>MPACCSWNDVFQYETNKVTRIQSVNYGTIKWILHMTVFSYVSFALMSDKLYQRKEPLISSVHTKVKGVAEVTENVTEGGVTKLVHGIFDTADYTLPLQGNSFFVMTNYLKSEGQEQKLCPEYPSRGKQCHSDQGCIKGWMDPQSKGIQTGRCIPYDQKRKTCEIFAWCPAEEGKEAPRPALLRSAENFTVLIKNNIDFPGHNYTTRNILPGMNISCTFHKTWNPQCPIFRLGDIFQEIGENFTEVAVQGGIMGIEIYWDCNLDSWSHRCQPKYSFRRLDDKYTNESLFPGYNFRYAKYYKENGMEKRTLIKAFGVRFDILVFGTGGKFDIIQLVVYIGSTLSYFGLATVCIDLIINTYASTCCRSRVYPSCKCCEPCAVNEYYYRKKCEPIVEPKPTLKYVSFVDEPHIWMVDQQLLGKSLQDVKGQEVPRPQTDFLELSRLSLSLHHSPPIPGQPEEMQLLQIEAVPRSRDSPDWCQCGNCLPSQLPENRRALEELCCRRKPGQCITTSELFSKIVLSREALQLLLLYQEPLLALEGEAINSKLRHCAYRSYATWRFVSQDMADFAILPSCCRWKIRKEFPKTQGQYSGFKYPY[3x]

P2X receptors (P2XRs) are trimeric, nonselective cation channels activated by adenosine triphosphate (ATP) that act as molecular sensors for extracellular ATP (eATP) (1–8). Predominantly expressed in immune cells, homomeric P2X7 receptors are molecular sensors for pathological inflammatory states by detecting and responding to mid-micromolar to low-millimolar local concentrations of eATP. P2X7 activation triggers signaling cascades that result in up-regulation of the NLRP3 (NOD-, LRR-, and pyrin domain–containing protein 3) inflammasome and activation of apoptotic pathways. Here, we report high-resolution cryo–electron microscopy structures of the homomeric rat P2X7 receptor bound to five previously known small-molecule allosteric antagonists and a sixth antagonist that we identify.

The structure of A438079-bound rP2X7 reveals the noncompetitive nature of this ligand, in contrast to previous data. Shallow binders, represented by A438079, A839977, AZD9056, and GSK1482160, extend minimally into the classical allosteric ligand-binding site. (A) Shallow binder A438079 occupies a shallow position in the classical allosteric ligand-binding site. Each ligand is located far from the other two symmetry-related molecules, preventing inter-ligand interactions. The structures of P2X7 in complex with the tetrazole-based antagonists, A438079 and A839977, provide some initial insights. Second, the additional rings found in A839977, but not A438079, participate in hydrophobic interactions at the entrance to the classical allosteric ligand-binding site. These two differences could possibly contribute to the slightly higher inhibitory potency of A839977 (IC50 = 116 ± 13 nM) compared to A438079 (IC50 = 550 ± 113 nM). The halogen atoms in A438079, A839977, and GSK1482160 all point toward A312. Following a 40-s exposure to an IC100 of antagonist, channel activity recovered more with exposure to AZD9056 and A438079 (82 ± 5% and 81 ± 5% of baseline current, respectively) when compared with exposure to A839977 and GSK1482160 (67 ± 6% and 69 ± 4% of baseline current, respectively). While A438079, AZD9056, and GSK1482160 demonstrated progressively less recovery after longer IC100 exposure times, none of these antagonists completely prevented channel recovery.> MAYRKRGARRETNLKQDDRMQEKEENKNVNTNSENKNATKPQLSEKVLSQKEEVITDNQEEIKIADEVKKSNKEESKQLLEVLKTKEEHQKEVQYEILQKTIPTFEPKESILKKLEDIKPEQVKKQTKLFRIFEPRQLPVYRANGEKELRNRWYWKLKRDTLPDGDYDVREYFLNLYDQVLTEMPDYLLLKDMAVENKNSRDAGKVVDSETAAICDAIFQDEETEGVVRRFIAEMRQRVQADRNVVNYPSILHPIDHAFNEYFLQHQLVEPLNNDIIFNYIPERIRNDVNYILNMDRNLPSTARYIRPN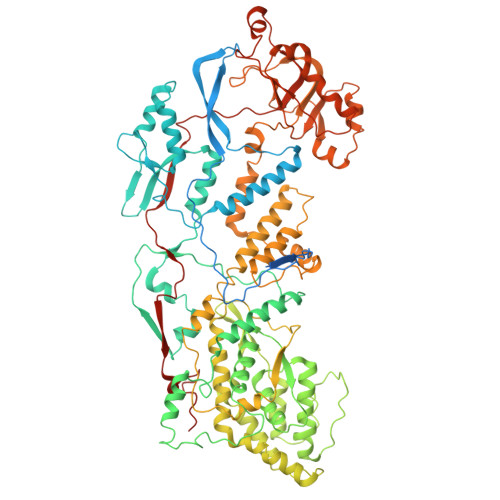LLQDRLNLHDNFESLWDTITTSNYILARSVVPDLKELVSTEAQIQKMSQDLQLEALTIQSETQFLTGINSQAANDCFKTLIAAMLSQRTMSLDFVTTNYMSLISGMWLLTVVPNDMFIRESLVACQLAIINTIIYPAFGMQRMHYRNGDPQTPFQIAEQQIQNFQVANWLHFVNNNQFRQVVIDGVLNQVLNDNIRNGHVVNQLMEALMQLSRQQFPTMPVDYKRSIQRGILLLSNRLGQLVDLTRLLAYNYETLMACITMNMQHVQTLTTEKLQLTSVTSLCMLIGNATVIPSPQTLFHYYNVNVNFHSNYNERINDAVAIITAANRLNLYQKKMKSIVEDFLKRLQIFDISRVPDDQMYRLRDRLRLLPVEIRRLDIFNLILMNMEQIERASDKIAQGVIIAYRDMQLERDEMYGYVNIARNLDGFQQINLEELMRTGDYAQITNMLLNNQPVALVGALPFITDSSVISLVAKLDATVFAQIVKLRKVDTLKPILYKINSDSNDFYLVANYDWVPTSTTKVYKQIPQQFDFRASMHMLTSNLTFTVYSDLLAFVSADTVEPINAVAFDNMRIMNEL>ETVSTQELYSIPEDQEPEDQEPEEPTPAPWARLWALQDGFANLECVNDNYWFGRDKSCEYCFDEPLLKRTDKYRTYSKKHFRIFREVGPKNSYIAYIEDHSGNGTFVNTELVGKGKRRPLNNNSEIALSLSRNKV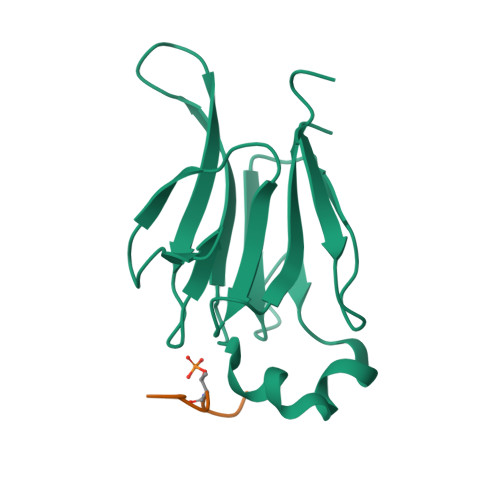FVFFDLTVDDQSVY[4x];>RHFDTYLIRR[4x]>MRRETVGEFSSDDDDDILLELGTRPPRFTQIPPSSAALQTQIPTTLEVTTTTLNNKQSKNDNQLVNQLNKAQGEASMLRDKINFLNIEREKEKNIQAVKVNELQVKHLQELAKLKQELQKLEDEKKFLQMEARGKSKREVITNVKPPSTTLSTNTNTITPDSSSVAIEAKPQSPQSKKRKISDNLLKKNMVPLNPNRIIPDETSLFLESILLHQIIGADLSTIEILNRLKLDYITEFKFKNFVIAKGAPIGKSIVSLLLRCKKTLTLDRFIDTLLEDIAVLIKEISVHPNESKLAVPFLVALMYQIVQFRPSATHNLALKDCFLFICDLIRIYHHVLKVPIHESNMNLHVEPQIFQYELIDYLIISYSFDLLEGILRVLQSHPKQTYMEFFDENILKSFEFVYKLALTISYKPMVNVIFSAVEVVNIITSIILNMDNSSDLKSLISGSWWRDCITRLYALLEKEIKSGDVYNENVDTTTLHMSKYHDFFGLIRNIGDNELGGLISKLIYTDRLQSVPRVISKEDIGMDSDKFTAPIIGYKMEKWLLKLKDEVLNIFENLLMIYGDDATIVNGEMLIHSSKFLSREQALMIERYVGQDSPNLDLRCHLIEHTLTIIYRLWKDHFKQLREEQIKQVESQLIMSLWRFLVCQTETVTANEREMRDHRHLVDSLHDLTIKDQASYYEDAFEDLPEYIEEELKMQLNKRTGRIMQVKYDEKFQEMARTILESKSFDLTTLEEADSLYISMGL[2x];>MESHVKYLDELILAIKDLNSGVDSKVQIKKVPTDPSSSQEYAKSLKILNTLIRNLKDQRRNNIMKNDTIFSKTVSALALLLEYNPFLLVMKDSNGNFEIQRLIDDFLNISVLNYDNYHRIWFMRRKLGSWCKACVEFYGKPAKFQLTAHFENTMNLYEQALTEVLLGKTELLKFYDTLKGLYILLYWFTSEYSTFGNSIAFLDSSLGFTKFDFNFQRLIRIVLYVFDSCELAALEYAEIQLKYISLVVDYVCNRTISTALDAPALVCCEQLKFVLTTMHHFLDNKYGLLDNDPTMAKGILRLYSLCISNDFSKCFVDHFPIDQWADFSQSEHFPFTQLTNKALSIVYFDLKRRSLPVEALKYDNKFNIWVYQSEPDSSLKNVTSPFDDRYKQLEKLRLLVLKKFNKTERGTLLKYRVNQLSPGFFQRAGNDFKLILNEASVSIQTCFKTNNITRLTSWTVILGRLACLESEKFSGTLPNSTKDMDNWYVCHLCDIEKTGNPFVRINPNRPEAAGKSEIFRILHSNFLSHPNIDEFSESLLSGILFSLHRIFSHFQPPKLTDGNGQINKSFKLVQKCFMNSNRYLRLLSTRIIPLFNISDSHNSEDEHTATLIKFLQSQKLPVVKENLVIAWTQLTLTTSNDVFDTLLLKLIDIFNSDDYSLRIMMTLQIKNMAKILKKTPYQLLSPILPVLLRQLGKNLVERKVGFQNLIELLGYSSKTILDIFQRYIIPYAIIQYKSDVLSEIAKIMCDGDTSLINQMKVNLLKKNSRQIFAVALVKHGLFSLDILETLFLNRAPTFDKGYITAYLPDYKTLAEITKLYKNSVTKDASDSENANMILCSLRFLITNFEKDKRHGSKYKNINNWTDDQEQAFQKKLQDNILGIFQVFSSDIHDVEGRTTYYEKLRVINGISFLIIYAPKKSIISALAQISICLQTGLGLKEVRYEAFRCWHLLVRHLNDEELSTVIDSLIAFILQKWSEFNGKLRNIVYSILDTLIKEKSDLILKLKPYTTLALVGKPELGILARDGQFARMVNKIRSTTDLIPIFANNLKSSNKYVINQNLDDIEVYLRRKQTERSIDFTPKKVGQTSDITLVLGALLDTSHKFRNLDKDLCEKCAKCISMIGVLDVTKHEFKRTTYSENEVYDLNDSVQTIKFLIWVINDILVPAFWQSENPSKQLFVALVIQESLKYCGLSSESWDMNHKELYPNEAKLWEKFNSVSKTTIYPLLSSLYLAQSWKEYVPLKYPSNNFKEGYKIWVKRFTLDLLKTGTTENHPLHVFSSLIREDDGSLSNFLLPYISLDIIIKAEKGTPYADILNGIIIEFDSIFTCNLEGMNNLQVDSLRMCYESIFRVFEYCKKWATEFKQNYSKLHGTFIIKDTKTTNMLLRIDEFLRTTPSDLLAQRSLETDSFERSALYLEQCYRQNPHDKNQNGQLLKNLQITYEEIGDIDSLDGVLRTFATGNLVSKIEELQYSENWKLAQDCFNVLGKFSDDPKTTTRMLKSMYDHQLYSQIISNSSFHSSDGKISLSPDVKEWYSIGLEAANLEGNVQTLKNWVEQIESLRNIDDREVLLQYNIAKALIAISNEDPLRTQKYIHNSFRLIGTNFITSSKETTLLKKQNLLMKLHSLYDLSFLSSAKDKFEYKSNTTILDYRMERIGADFVPNHYILSMRKSFDQLKMNEQADADLGKTFFTLAQLARNNARLDIASESLMHCLERRLPQAELEFAEILWKQGENDRALKIVQEIHEKYQENSSVNARDRAAVLLKFTEWLDLSNNSASEQIIKQYQDIFQIDSKWDKPYYSIGLYYSRLLERKKAEGYITNGRFEYRAISYFLLAFEKNTAKVRENLPKVITFWLDIAAASISEAPGNRKEMLSKATEDICSHVEEALQHCPTYIWYFVLTQLLSRLLHSHQSSAQIIMHILLSLAVEYPSHILWYITALVNSNSSKRVLRGKHILEKYRQHSQNPHDLVSSALDLTKALTRVCLQDVKSITSRSGKSLEKDFKFDMNVAPSAMVVPVRKNLDIISPLESNSMRGYQPFRPVVSIIRFGSSYKVFSSLKKPKQLNIIGSDGNIYGIMCKKEDVRQDNQYMQFATTMDFLLSKDIASRKRSLGINIYSVLS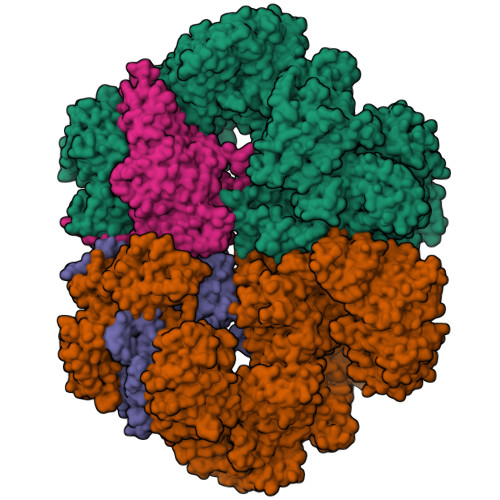LREDCGILEMVPNVVTLRSILSTKYESLKIKYSLKSLHDRWQHTAVDGKLEFYMEQVDKFPPILYQWFLENFPDPINWFNARNTYARSYAVMAMVGHILGLGDRHCENILLDIQTGKVLHVDFDCLFEKGKRLPVPEIVPFRLTPNLLDALGIIGTEGTFKKSSEVTLALMRKNEVALMNVIETIMYDRNMDHSIQKALKVLRNKIRGIDPQDGLVLSVAGQTETLIQEATSEDNLSKMYIGWLPFW[2x]> GSFTDSPPERQIVVGICSMAKKSKSKPMKEILERISLFKYITVVVFEEEVILNEPVENWPLCDCLISFHSKGFPLDKAVAYAKLRNPFVINDLNMQYLIQDRREVYSILQAEGILLPRYAILNRDPNNPKECNLIEGEDHVEVNGEVFQKPFVEKPVSAEDHNVYIYYPTSAGGGSQRLFRKIGSRSSVYSPESNVRKTGSYIYEEFMPTDGTDVKVYTVGPDYAHAEARKSPALDGKVERDSEGKEVRYPVILNAREKLIAWKVCLAFKQTVCGFDLLRANGQSYVCDVNGFSFVKNSMKYYDDCAKILGNIVMRELAPQFHIPWSI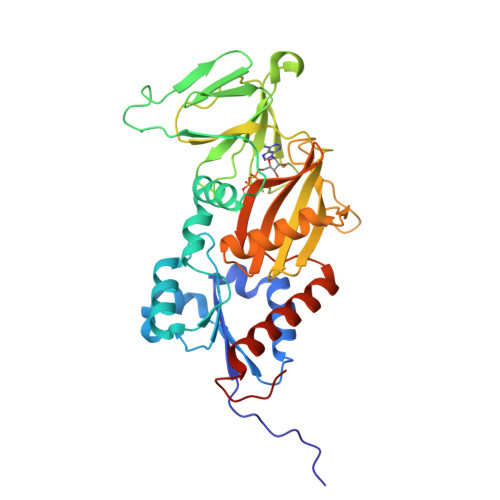PLEAED> SMSVKKPKRDDSKDLALCSMILTEMETHEDAWPFLLPVNLKLVPGYKKVIKKPMDFST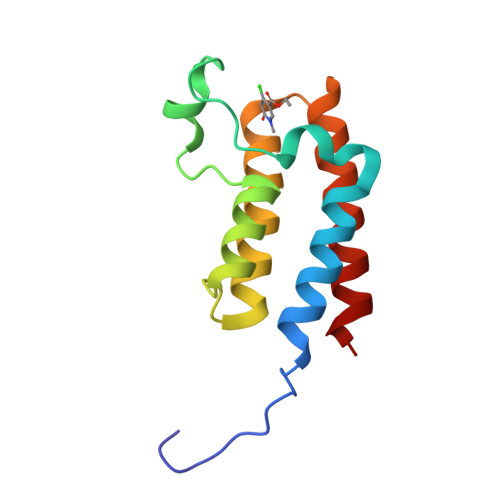IREKLSSGQYPNLETFALDVRLVFDNCETFNEDDSDIGRAGHNMRKYFEKKWTDTFKV(2~{R},4~{S})-4-[bis(fluoranyl)methoxy]-~{N}-methyl-1-(2~{H}-pyrazolo[4,3-b]pyridin-6-ylcarbonyl)pyrrolidine-2-carboxamide | C14 H15 F2 N5 O3 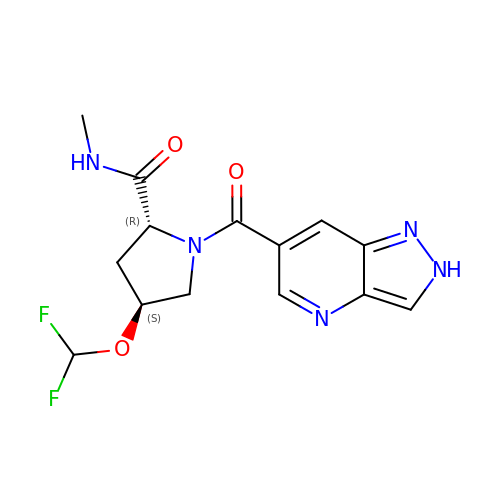| IIQVNHRKCWVSPV-GZMMTYOYSA-N>[2x]MVMSIEYKSEAAAVRRFPGSIVVMGVSGSGKSSVGEAIAEACGYPFIEGD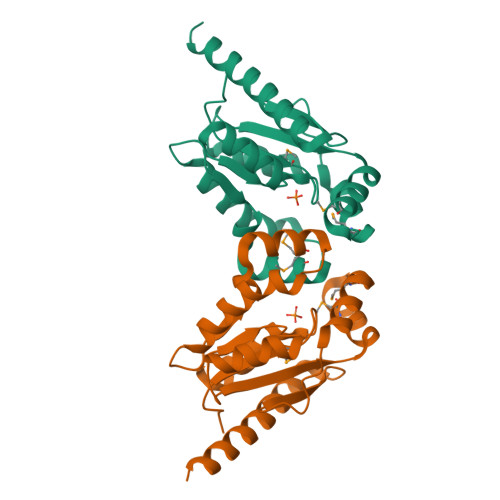ALHPPENIRKMSEGIPLTDDDRWPWLAAIGERLASREPVVVSCSALKRSYRDKLRESAPGGLAFVFLHGSESVLAERMHHRTGHFMPSSLLQTQLETLEDPRGEVRTVAVDVAQPLAEIVREALAGLARLAENLYFQSHHHHHHWSHPQFEK> MSVTTLGQSFPANAKVKYYYKLSEKQDLDAFVNSIFVGSYKLKQISYLLYGNTKIVSAPVV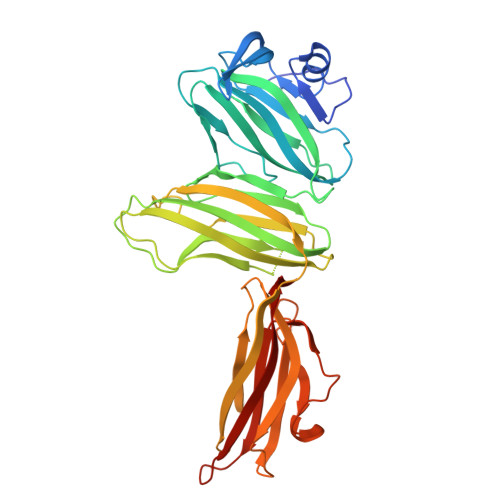PLGPNASIIIDDELQEGLYLIRIKVYNTNSFSVTVTPFFNNNNTMTYSIGANSEFEIYDIFTKEQGNIYYIQLPPGLAILEFSLERVFEKGNRINIPKIIHTSGNGYISFRLRKGTYAIKMPYSYNNTTSTTFTNFQFGTISTSVATIPLVISSIPANGSGSGTFLVYLKITGDYEDVKFSVTYGGGLGVPFTFGLEVEEINELVENTNFVTQSVTLSGSQVTQSILNVQGSGSHLRLKYASVSGLTTAVTQCQLQATNLNRSTTYSTVWDFIAGGSSTPPSWDIREINSIQLVANGGSSTSSVTITLILVYEQIAGELS>[2x]MNSPQNVSTKKVTVTGAAGQISYSLLWRIANGEVFGTDTPVELKLLEIPQALGGAEGVAMELLDSAFPLLRNITITADA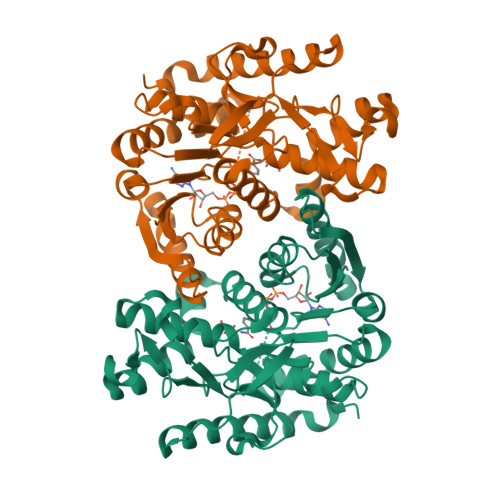NEAFDGANAAFLVGAKPRGKGEERADLLANNGKIFGPQGKAINDNAADDIRVLVVGNPANTNALIASAAAPDVPASRFNAMMRLDHNRAISQLATKLGRGSAEFNNIVVWGNHSATQFPDITYATVGGEKVTDLVDHDWYVEEFIPRVANRGAEIIEVRGKSSAASAASSAIDHMRDWVQGTEAWSSAAIPSTGAYGIPEGIFVGLPTVSRNGEWEIVEGLEISDFQRARIDANAQELQAEREAVRDLLLEHHHHHH> MKFSAKRLPSTRLGTFLENRVNDFLRRQNHPESGEVTVRVVHASDKTVEVKPGMKARFVDSGEMAESFPYRTKALFAFEEIDGVDLCFFGMHVQEYGSDCPPPNQRRVYISYLDSVHF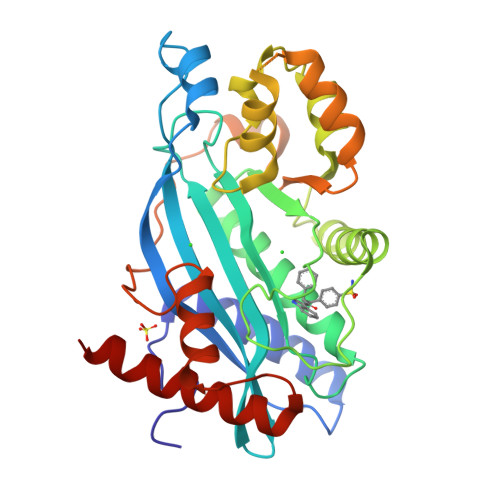FRPKCLRTAVYHEILIGYLEYVKKLGYTTGHIWACPPSEGDDYIFHCHPPDQKIPKPKRLQEWYKKMLDKAVSERIVHDYKDIFKQATEDRLTSAKELPYFEGDFWPNVLEESIKELEQKTSKNKSSLSRGNKKKPGMPNVSNDLSQKLYATMEKHKEVFFVIRLIAGPAANSLPPIVDPDPLIPCDLMDGRDAFLTLARDKHLEFSSLRRAQWSTGCMLVELHTQSQDRF> MVVLDKKLLERLTSRKVPLEELEDMEKKCFLSTFTYQDAFDLGTYIKNAVKENFPDKPVAIDISLPNGHCLFRTVTYGGSALDN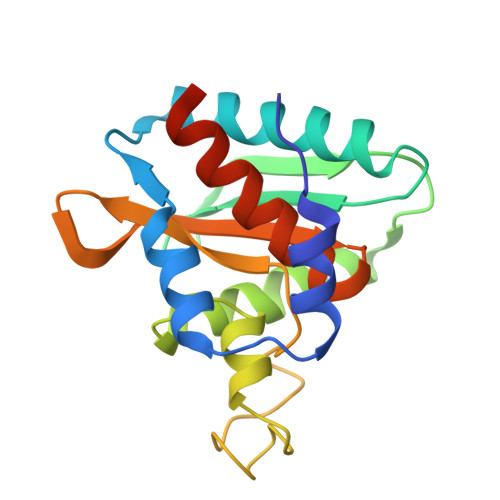DFWIQRKKKTALRFGHSSFYMGCKKGDKTPEEKFFVDSKEYAFHGGAVLIQSERSTYPYACLTISGLKQEEDHLMAVSSLIAFANESLEEDLNLD> ASNLKIVRMDRTAGCVTGGEEIYLLCDKVQKDDIQIRFYEEEENGGVWEGFG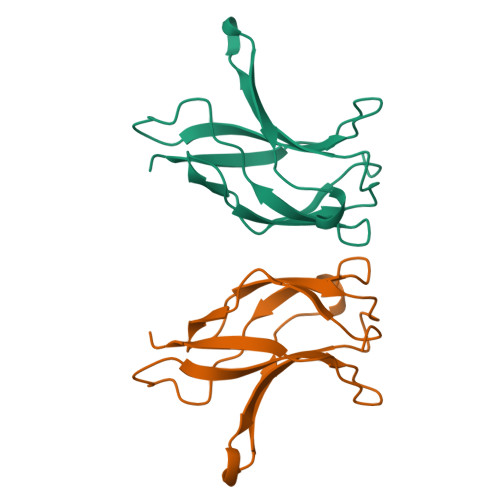DFSPTDVHRQFAIVFKTPKYKDVNITKPASVFVQLRRKSDLETSEPKPFLYYPE>MKLSLMVAISKNGVIGNGPDIPWSAKGEQLLFKAITYNQWLLVGRKTFESMGALPNRKYAVVTRSSFTSDNENVLIFPSIKDALTNLKKITDHVIVSGGGEIYKSLIDQVDTLHISTIDIEPEGDVYFPEIPSNFRPVFTQDFASNINYSYQIWQKGLEHH[6x]

Two plasmid-encoded dihydrofolate reductase (DHFR) isoforms, DfrA1 and DfrA5, that give rise to high levels of resistance in Gram-negative bacteria were structurally and biochemically characterized to reveal the mechanism of TMP resistance and to support phylogenic groupings for drug development against antibiotic resistant pathogens. TMP is a selective inhibitor of bacterial dihydrofolate reductase (DHFR), which catalyzes the NADPH-dependent reduction of dihydrofolate (DHF) to tetrahydrofolate (THF), a necessary step for the recycling of reduced folate cofactors. Trimethoprim resistance in Enterobacteriaceae occurs almost exclusively through the acquisition of plasmid-associated dfr genes that encode intrinsically insensitive DHFR enzymes. Expectedly, all three enzymes form the stereotypical DHFR fold with an eight-stranded β-sheet, four α-helices (B, C, E, and F) and three catalytic loops (the Met20, F-G, and G-H loops).

The crystal structure of DfrA1:TMP, determined to 2.2 Å, shows the antifolate interactions in the active site more closely resemble the binding mode observed in DfrA5 than in EcDHFR. Similarly, electrostatic interactions between Glu28DfrA1 and the diaminopyrimidine ring dictate the ligand binding mode. Additionally, critical hydrophobic contacts are lost through the L28Q substitution. Excitingly, there are structural differences that rationalize the higher levels of TMP-resistance observed with DfrA1 compared to DfrA5. In DfrA1, a bridging water molecule facilitates the interaction between Glu28 and TMP, representing a loss of direct H-bond interactions. Another pronounced difference between the DfrA1:TMP and DfrA5:NADPH:TMP complexes is seen in the Met20 loop. In the DfrA1:TMP complex, this loop takes on a conformation reminiscent of the EcDHFR occluded conformation with the Met20 loop occupying the NADPH binding site. The direct effect on TMP binding is through interactions with Met16DfrA1 that result in a 2 Å push and ~90° rotation of the trimethoxyphenyl group as compared to the DfrA5:NADPH:TMP structure, correlating with a >3-fold increase in resistance between the two enzymes. Moreover, binding of TMP reorganizes DfrA1 into a conformation similar to the occluded conformation of EcDHFR that involves a notable shift of the Met20 loop. Of the ~500 structures of DHFR from various organisms available in the PDB, this is the first isoform of DHFR evolutionarily distinct from EcDHFR reported in the occluded state.> GSPEFEKVRIYRMDGSYRSVELKHGNNTTVQQIMEGMRLSQETQQYFTIWI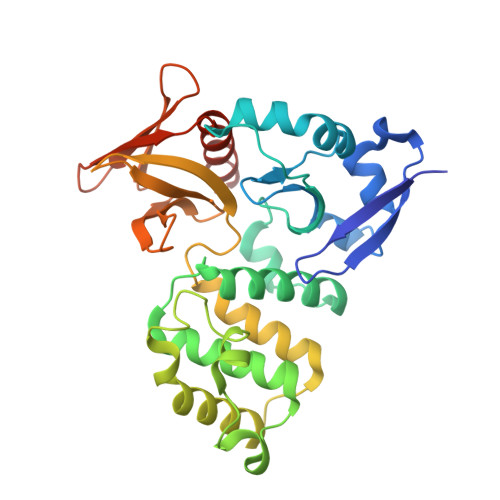CSENLSLQLKPYHKPLQHVRDWPEILAELTNLDPQRETPQLFLRRDVRLPLEVEKQIEDPLAILILFDEARYNLLKGFYTAPDAKLITLASLLLQIVYGNYESKKHKQGFLNEENLKSIVPVTKLKSKAPHWTNRILHEYKNLSTSEGVSKEMHHLQRMFLQNCWEIPTYGAAFFTGQIFTKASPSNHKVIPVYVGVNIKGLHLLNMETKALLISLKYGCFMWQLGDTDTCFQIHSMENKMSFIVHTKQAGLVVKLLMKLNGQLMPTERNS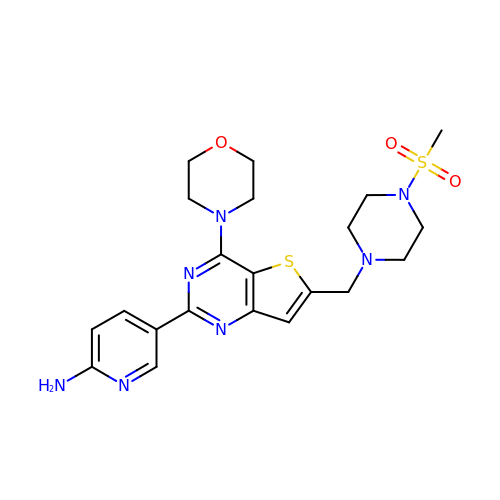5-(6-{[4-(methylsulfonyl)piperazin-1-yl]methyl}-4-morpholin-4-ylthieno[3,2-d]pyrimidin-2-yl)pyridin-2-amine | C21 H27 N7 O3 S2 | JEHTXQHLTKVUGY-UHFFFAOYSA-N> RTFDLEEKLQTNKYNANFVTFMEGKDFNVEYIQRGGLRDPLIFKNSDGLGIKMPDPDFTVNDVKMCVGSR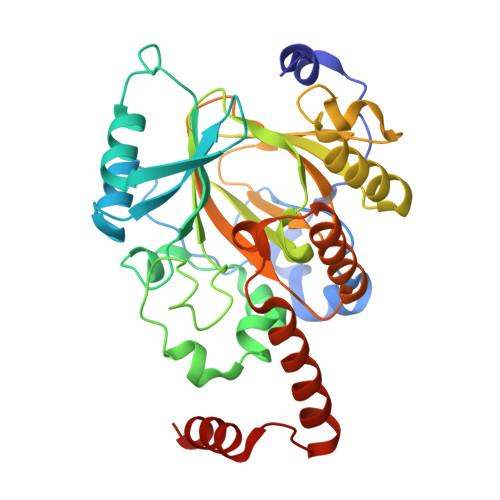RMVDVMDVNTQKGIEMTMAQWTRYYETPEEEREKLYNVISLEFSHTRLENMVQRPSTVDFIDWVDNMWPRHLKESQTESTNAILEMQYPKVQKYCLMSVRGCYTDFHVDFGGTSVWYHIHQGGKVFWLIPPTAHNLELYENWLLSGKQGDIFLGDRVSDCQRIELKQGYTFVIPSGWIHAVYTPTDTLVFGGNFLHSFNIPMQLKIYSIEDRTRVPNKFRYPFYYEMCWYVLERYVYCITNRSHLTKDFQKESLSMDME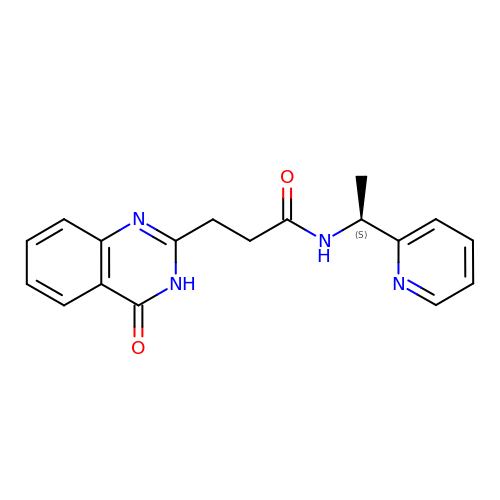3-(4-oxo-3,4-dihydroquinazolin-2-yl)-N-[(1S)-1-(pyridin-2-yl)ethyl]propanamide | C18 H18 N4 O2 | HWTVYWVFOWWESR-LBPRGKRZSA-N>GSHMGEIRPTIGQQMETGDQRFGDLVFRQLAPNVWQHTSYLDMPGFGAVASNGLIVRDGGRVLVVDTAWTDDQTAQILNWIKQEINLPVALAVVTHAHQDKMGGMDALHAAGIATYANALSNQLAPQEGMVAAQHSLTFAANGWVEPATAPNFGPLKVFYPGPGHTSDNITVGIDGTDIAFGGCLIKDSKAKSLGNLGDADTEHYAASARAFGAAFPKASMIVMSHSAPDSRAAITHTARMADKLR[2x]

Production of metallo-β-lactamases (MBLs), which hydrolyze carbapenems, is a cause of carbapenem resistance in Enterobacteriaceae. The genes encoding MBLs, including IMP, NDM, and VIM types, have become widely prevalent via bacterium-specific transferable genetic apparatuses such as plasmids. We report here that sulfamoyl heteroarylcarboxylic acids (SHCs) can competitively inhibit the globally spreading and clinically relevant MBLs (i.e., IMP-, NDM-, and VIM-type MBLs) at nanomolar to micromolar orders of magnitude. X-ray crystallographic analyses revealed the inhibition mode of SHCs against MBLs; the sulfamoyl group of SHCs coordinated to two zinc ions, and the carboxylate group coordinated to one zinc ion and bound to positively charged amino acids Lys224/Arg228 conserved in MBLs.

The modes of interaction between SFC and NDM-1/VIM-2 were also determined. The key aspects for binding through the sulfamoyl and carboxylate groups in NDM-1–SFC and VIM-2–SFC structures were quite similar to those determined for the IMP-1–SFC structure. The sulfamoyl group coordinates to Zn1 and Zn2, the carboxylate oxygen O1 coordinates to Zn2, and the other carboxylate oxygen O2 binds to Asn233 and Lys224 (NDM-1)/Arg228 (VIM-2). Of note, there was no corresponding stabilization caused by Trp64 in the L3 loop of IMP-1, which holds SFC in the active site, in both NDM-1–SFC and VIM-2–SFC structures. Such structural differences in the L3 loop may cause differences in SFC affinity; the Ki values determined for inhibition of NDM-1 and VIM-2 by SFC were 9.82 μM and 2.81 μM, respectively, which are >10-fold higher than that of IMP-1 (0.22 μM). Although the inhibitory activities of SFC differed with individual MBLs, SFC bound to MBLs via their common architectures, through Zn1, Zn2, and Asn233, and through positively charged basic residue Lys224 or Arg228 of the L10 loop.> HGSMKEFYLTVEQIGDSIFERYIDSNGRERTREVEYKPSLFAHCPESQATKYFDIYGKPCTRKLFANMRDASQWIKRMEDIGLEALGMDDFKLAYLSDTYNYEIKYDHTKIRVANFDIEVTSPDGFPEPSQAKHPIDAITHYDSIDDRFYVFDLLNSPYGNVEEWSIEIAAKLQEQGGDEVPSEIIDKIIYMPFDNEKELLMEYLNFWQQKTPVILTGWNVESFAIPYVYNRIKNIFGESTAKRLSPHRKTRVKVIENMYGSREIITLFGISVLDYIDLYKKFSFTNQPSYSLDYISEFELNVGKLKYDGPISKLRESNHQRYISYNIIAVYRVLQIDAKRQFINLSLDMGYYAKIQIQSVFSPIKTWDAIIFNSLKEQNKVIPQGRSHPVQPYPGAFVKEPIPNRYKYVMSFDLTSLYPSIIRQVNISPETIAGTFKVAPLHDYINAVAERPSDVYSCSPNGMMYYKDRDGVVPTEITKVFNQRKEHKGYMLAAQRNGEIIKEALHNPNLSVDEPLDVDYRFDFSDEIKEKIKKLSAKSLNEMLFRAQRTEVAGMTAQINRKLLINSLYGALGNVWFRYYDLRNATAITTFGQMALQWIERKVNEYLNEVCGTEGEAFVLY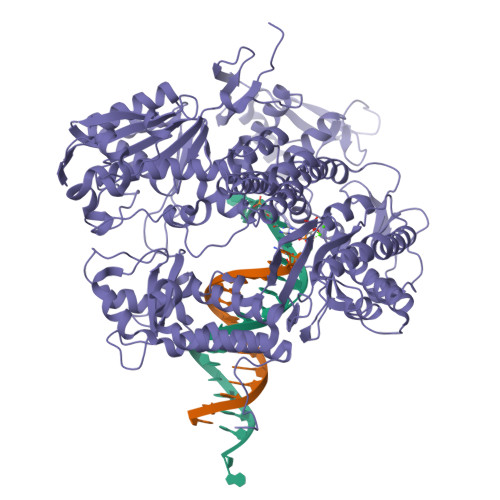GDTDSIYVSADKIIDKVGESKFRDTNHWVDFLDKFARERMEPAIDRGFREMCEYMNNKQHLMFMDREAIAGPPLGSKGIGGFWTGKKRYALNVWDMEGTRYAEPKLKIMGLETQKSSTPKAVQKALKECIRRMLQEGEESLQEYFKEFEKEFRQLNYISIASVSSANNIAKYDVGGFPGPKCPFHIRGILTYNRAIKGNIDAPQVVEGEKVYVLPLREGNPFGDKCIAWPSGTEITDLIKDDVLHWMDYTVLLEKTFIKPLEGFTSAAKLDYEKKASLFDMFDF>AGENGATTTFDGPVAAERFSADTTLEAAFLKTTSETNHAATIYQAGTSGDGAALNVISDNPGTSAMYLSGTETARGTLKITHRGYADGSDKDAAALSLDLRVAGTAAQGIYVTATNGPTKGNLIALRNNTGLDDFVVKGTGRIGVGIDRAATPRAQVHIVQRGDALAALLVEGSVRIGNAATVPTSVDSSGGGALYASGGALLWRGSNGTVTTI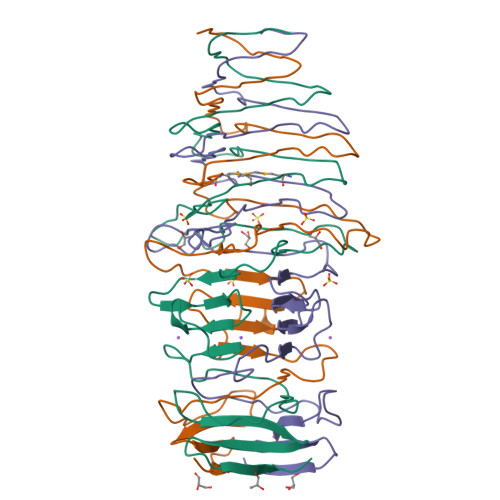APA[2x]>SNAALKLMQYIGDAIGTIRDPQELFRTVTDKLRLLFAFDSAVIITIDRERREASVFFEMLRFELPEQLRHQTRSIAGTWLEGHLDDRTVTVASIARDIPSFGADGAPLLWTLHELGMRQIVLSPLRSGGRVIGFLSFVSAEEKLWSDGDKSLL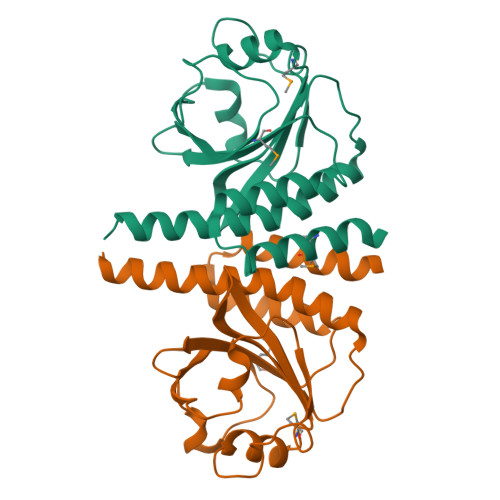SGVSSSIAIAVSNALAYEELRQRE[2x]4-[(2-bromo-2-methylpropanoyl)amino]-L-phenylalanine | C13 H17 Br N2 O3 | 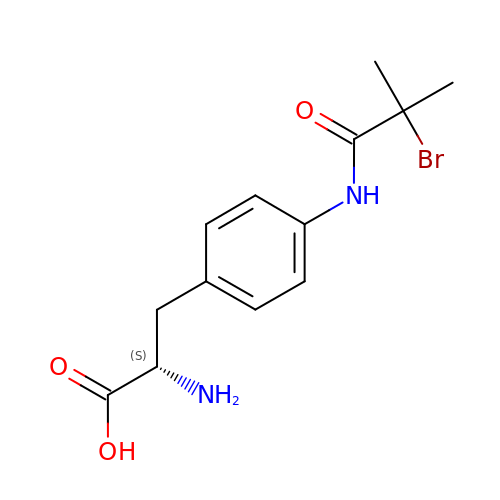ZKDRICVKKZOGNC-JTQLQIEISA-N>XGEIAQAIKEIAKAIKEVAWAFKEIAQAIKGX[2x]

To address this, here we describe the design, characterization, and application of small-molecule:peptide ternary complexes in aqueous solution. This uses α-helical barrel (αHB) peptide assemblies, which comprise 5 or more α helices arranged around central channels. The αHBs present interesting de novo scaffolds because of their stability, controllable oligomeric states and lumen sizes, robustness to mutation, and the potential to functionalize the internal channels for small-molecule binding and catalysis by incorporating both proteinogenic and noncanonical amino acids. We have demonstrated the ability of the lumens of de novo designed α-helical barrel assemblies (αHBs) to bind and organize two ligands in conformations that accelerate the time scales for two different photoinduced chemical processes.

For simplicity, henceforth we refer to the three αHB peptides CC-Type2-[SgLaId], CC-Type2-[IaVd] and CC-Type2-[IaId]–I17V-I21F, as the hexamer, heptamer and octamer, respectively. Finally, we used analytical ultracentrifugation to confirm that the oligomeric states of the barrels with bound ligand matched those observed by crystallography. Using ultrafast spectroscopy, we demonstrate that the channels of heptameric and octameric peptide assemblies are long enough to encapsulate both dyes simultaneously, and wide enough to juxtapose them for efficient energy transfer on picosecond time scales. Analysis of these data yielded FRET time constants of 0.98 ± 0.2 ns for the heptamer and 1.3 ± 0.2 ns for the octamer. Using the Förster equation (eq S6), the internuclear distance between DPH and Nile red was estimated as 3.3–3.9 nm for the heptamer, and 3.1–3.9 nm for the octamer. These are well within the length of the hydrophobic channels at ∼4.6 nm and demonstrate successful encapsulation of both DPH and Nile red within the same barrel. Analysis of the data returned fast energy transfer time constants between DPH and Nile red: 10.4 ± 2.4 ps in the heptamer, and 7.9 ± 5.7 ps in the octamer, reconciling the high energy transfer efficiency determined from steady state emission measurements. For the octamer, we observed a broad global minimum at 4.1 Å and a shallower minimum around 20 Å. We also tested the octamer in this reaction, although docking predicted that its channel should be too wide for precise anthracene π-stacking. Consistent with this, while the octamer did promote the conversion, the loss of anthracene fluorescence signal was linear, slower than with the heptamer, and similar to the controls.Transcription factor (TF) IIIC, a six-subunit protein complex with a molecular weight (MW) of 624 kDa in humans, facilitates transcription of type 1 (5S ribosomal RNA) and type 2 [e.g., transfer RNAs (tRNAs)] RNA polymerase (Pol) III target genes. TFIIIC is composed of two subcomplexes, τA and τB, that bind two gene internal DNA motifs: A-box and B-box. τA binds the A-box with low affinity and is required to recruit TFIIIB to the promoter DNA. τB interacts with the B-box with high affinity and, therefore, is essential for target DNA recognition of type 2 genes. hTFIIIC consists of τA subunits TFIIIC35, TFIIIC63, and TFIIIC102 and τB subunits TFIIIC90, TFIIIC110, and TFIIIC220. TFIIIC220 forms an integral part of both τA and τB connecting the two subcomplexes via a ~550–amino acid residue flexible linker.

Our cryo-EM analysis yielded a high-resolution structure of human τA, which, however, remained in the DNA-unbound state in the presence of the tRNA gene. This observation is in agreement with biochemical studies on hTFIIIC, where the TFIIIC2 component interacts exclusively with B-box and is deficient in interacting with A-box. When inspecting the 3D reconstruction of human τA, we found that 50% of the cryo-EM density corresponds to the τA subunits TFIIIC35, TFIIIC63, and TFIIIC102 (τ55, τ95, and τ131 in yeast). TFIIIC35-TFIIIC63 form a heterodimer that binds the C-terminal TPR domain of TFIIIC102. Unexpectedly, the remaining ~50% of the cryo-EM density belongs to the C-terminal half of the τB subunit TFIIIC220. The C-terminal half of TFIIIC220 forms an integral part of human τA, suggesting that TFIIIC220 links τA and τB with a ~550-residue-long linker between its N and C termini. Whereas the N-terminal WH1 to WH4 and eWH domains either directly or indirectly (WH1) mediate B-box recognition, the C-terminal WH5 to WH8 domains form an integral part of τA and, thereby, serve as a hook that tethers τA and τB. A potential reason why we captured human τA exclusively in the DNA-unbound state could be due to posttranslational modifications that may regulate the affinity of τA to the A-box motif. An alternative explanation is that human τA mainly did not bind the A-box due to the absence of TFIIIB. Once TFIIIC is anchored to the tRNA gene, the τA subcomplex, connected by a ~550–amino acid (aa) flexible linker to τB, will search for the A-box motif, separated from the B-box with a variable distance between 30 and 67 bp, by a fly-casting mechanism.

> MDALESLLDEVALEGLDGLCLPALWSRLETRVPPFPLPLEPCTQEFLWRALATHPGISFYEEPRERPDLQLQDRYEEIDLETGILESRRDPVALEDVYPIHMILENKDGIQGSCRYFKERKNITNDIRTKSLQPRCTMVEAFDRWGKKLIIVASQAMRYRALIGQEGDPDLKLPDFSYCILERLGRSRWQGELQRDLHTTAFKVDAGKLHYHRKILNKNGLITMQSHVIRLPTGAQQHSILLLLNRFHVDRRSKYDILMEKLSVMLSTRTNHIETLGKLREELGLCERTFKRLYQYMLNAGLAKVVSLRLQEIHPECGPCKTKKGTDVMVRCLKLLKEFKRNDHDDDEDEEVISKTVPPVDIVFERDMLTQTYDLIERRGTKGISQAEIRVAMNVGKLEARMLCRLLQRFKVVKGFMEDEGRQRTTKYISCVFAEESDLSRQYQREKARSELLTTVSLASMQEESLLPEGEDTFLSESDSEEERSSSKRRGRGSQKDTRASANLRPKTQPHHSTPTKGGWKVVNLHPLKKQPPSFPGAAEERACQSLASRDSLLDTSSVSEPNVSFVSHCADSNSGDIAVIEEVRMENPKESSSSLKTGRHSSGQDKPHETYRLLKRRNLIIEAVTNLRLIESLFTIQKMIMDQEKQEGVSTKCCKKSIVRLVRNLSEEGLLRLYRTTVIQDGIKKKVDLVVHPSMDQNDPLVRSAIEQVRFRISNSSTANRVKTSQPPVPQGEAEEDSQGKEGPSGSGDSQLSASSRSESGRMKKSDNKMGITPLRNYHPIVVPGLGRSLGFLPKMPRLRVVHMFLWYLIYGHPASNTVEKPSFISERRTIKQESGRAGVRPSSSGSAWEACSEAPSKGSQDGVTWEAEVELATETVYVDDASWMRYIPPIPVHRDFGFGWALVSDILLCLPLSIFIQIVQVSYKVDNLEEFLNDPLKKHTLIRFLPRPIRQQLLYKRRYIFSVVENLQRLCYMGLLQFGPTEKFQDKDQVFIFLKKNAVIVDTTICDPHYNLARSSRPFERRLYVLNSMQDVENYWFDLQCVCLNTPLGVVRCPRVRKNSSTDQGSDEEGSLQKEQESAMDKHNLERKCAMLEYTTGSREVVDEGLIPGDGLGAAGLDSSFYGHLKRNWIWTSYIINQAKKENTAAENGLTVRLQTFLSKRPMPLSARGNSRLNIWGEARVGSELCAGWEEQFEVDREPSLDRNRRVRGGKSQKRKRLKKDPGKKIKRKKKGEFPGEKSKRLRYHDEADQSALQRMTRLRVTWSMQEDGLLVLCRIASNVLNTKVKGPFVTWQVVRDILHATFEESLDKTSHSVGRRARYIVKNPQAYLNYKVCLAEVYQDKALVGDFMNRRGDYDDPKVCANEFKEFVEKLKEKFSSALRNSNLEIPDTLQELFARYRVLAIGDEKDQTRKEDELNSVDDIHFLVLQNLIQSTLALSDSQMKSYQSFQTFRLYREYKDHVLVKAFMECQKRSLVNRRRVNHTLGPKKNRALPFVPMSYQLSQTYYRIFTWRFPSTICTESFQFLDRMRAAGKLDQPDRFSFKDQDNNEPTNDMVAFSLDGPGGNCVAVLTLFSLGLISVDVRIPEQIIVVDSSMVENEVIKSLGKDGSLEDDEDEEDDLDEGVGGKRRSMEVKPAQASHTNYLLMRGYYSPGIVSTRNLNPNDSIVVNSCQMKFQLRCTPVPARLRPAAAPLEELTMGTSCLPDTFTKLINPQENTCSLEEFVLQLELSGYSPEDLTAALEILEAIIATGCFGIDKEELRRRFSALEKAGGGRTRTFADCIQALLEQHQVLEVGGNTARLVAMGSAWPWLLHSVRLKDREDADIQREDPQARPLEGSSSEDSPPEGQAPPSHSPRGTKRRASWASENGETDAEGTQMTPAKRPALQDSNLAPSLGPGAEDGAEAQAPSPPPALEDTAAAGAAQEDQEGVGEFSSPGQEQLSGQAQPPEGSEDPRGFTESFGAANISQAARERDCESVCFIGRPWRVVDGHLNLPVCKGMMEAMLYHIMTRPGIPESSLLRHYQGVLQPVAVLELLQGLESLGCIRKRWLRKPRPVSLFSTPVVEEVEVPSSLDESPMAFYEPTLDCTLRLGRVFPHEVNWNKWIHLGGGSGGGSGGSLEVLFQGPGSGSDYKDDDDKGDYKDDDDKGDYKDDDDK;> MSGFSPELIDYLEGKISFEEFERRREERKTREKKSLQEKGKLSAEENPDDSEVPSSSGINSTKSQDKDVNEGETSDGVRKSVHKVFASMLGENEDDEEEEEEEEEEEEEEETPEQPTAGDVFVLEMVLNRETKKMMKEKRPRSKLPRALRGLMGEANIRFARGEREEAILMCMEIIRQAPLAYEPFSTLAMIYEDQGDMEKSLQFELIAAHLNPSDTEEWVRLAEMSLEQDNIKQAIFCYTKALKYEPTNVRYLWERSSLYEQMGDHKMAMDGYRRILNLLSPSDGERFMQLARDMAKSYYEANDVTSAINIIDEAFSKHQGLVSMEDVNIAAELYISNKQYDKALEIITDFSGIVLEKKTSEEGTSEENKAPENVTCTIPDGVPIDITVKLMVCLVHLNILEPLNPLLTTLVEQNPEDMGDLYLDVAEAFLDVGEYNSALPLLSALVCSERYNLAVVWLRHAECLKALGYMERAAESYGKVVDLAPLHLDARISLSTLQQQLGQPEKALEALEPMYDPDTLAQDANAAQQELKLLLHRSTLLFSQGKMYGYVDTLLTMLAMLLKVAMNRAQVCLISSSKSGERHLYLIKVSRDKISDSNDQESANCDAKAIFAVLTSVLTKDDWWNLLLKAIYSLCDLSRFQEAELLVDSSLEYYSFYDDRQKRKELEYFGLSAAILDKNFRKAYNYIRIMVMENVNKPQLWNIFNQVTMHSQDVRHHRFCLRLMLKNPENHALCVLNGHNAFVSGSFKHALGQYVQAFRTHPDEPLYSFCIGLTFIHMASQKYVLRRHALIVQGFSFLNRYLSLRGPCQESFYNLGRGLHQLGLIHLAIHYYQKALELPPLVVEGIELDQLDLRRDIAYNLSLIYQSSGNTGMAQTLLYTYCSI;> MHHHHHHENLYFQGMAAEAADLGLGAAVPVELRRERRMVCVEYPGVVRDVAKMLPTLGGEEGVSRIYADPTKRLELYFRPKDPYCHPVCANRFSTSSLLLRIRKRTRRQKGVLGTEAHSEVTFDMEILGIISTIYKFQGMSDFQYLAVHTEAGGKHTSMYDKVLMLRPEKEAFFHQELPLYIPPPIFSRLDAPVDYFYRPETQHREGYNNPPISGENLIGLSRARRPHNAIFVNFEDEEVPKQPLEAAAQTWRRVCTNPVDRKVEEELRKLFDIRPIWSRNAVKANISVHPDKLKVLLPFIAYYMITGPWRSLWIRFGYDPRKNPDAKIYQVLDFRIRCGMKHGYAPSDLPVKAKRSTYNYSLPITVKKTSSQLVTMHDLKQGLGPSGTSGARKPASSKYKLKDSVYIFREGALPPYRQMFYQLCDLNVEELQKIIHRNDGAENSCTERDGWCLPKTSDELRDTMSLMIRQTIRSKRPALFSSSAKADGGKEQLTYESGEDEEDEEEEEEEEEDFKPSDGSENEMETEILDYV;> MAAAADERSPEDGEDEEEEEQLVLVELSGIIDSDFLSKCENKCKVLGIDTERPILQVDSCVFAGEYEDTLGTCVIFEENVEHADTEGNNKTVLKYKCHTMKKLSMTRTLLTEKKEGEENIGGVEWLQIKDNDFSYRPNMICNFLHENEDEEVVASAPDKSLELEEEEIQMNDSSNLSCEQEKPMHLEIEDSGPLIDIPSETEGSVFMETQMLP>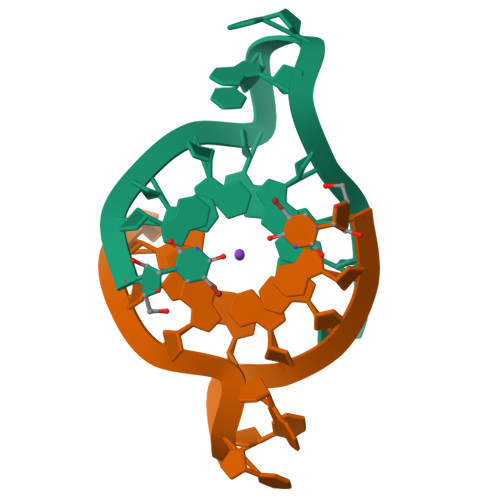UAGGGUUAGGGU[2x]> MLIRRLKDARLRAGISQEKLGVLAGIDEASASARMNQYEKGKHAPDFEMANRLAKVLKIPVSYLYTPEDDLAQIILTWNELNEQERKRINFYIRKKAK

Controller proteins play a key role in the temporal regulation of gene expression in bacterial restriction–modification (R–M) systems and are important mediators of horizontal gene transfer. They form the basis of a highly cooperative, concentration-dependent genetic switch involved in both activation and repression of R–M genes. Here we present biophysical, biochemical, and high-resolution structural analysis of a novel class of controller proteins, exemplified by C.Csp231I. In contrast to all previously solved C-protein structures, each protein subunit has two extra helices at the C-terminus, which play a large part in maintaining the dimer interface.

The protein crystallised in two space groups: a monoclinic form (P21) and a cubic form (F4132). The calculated Matthews coefficients were 2.38 Å3 Da− 1 (one monomer in the asymmetric unit) and 2.01 Å3 Da− 1 (two monomers in the asymmetric unit) for the cubic and monoclinic structures, respectively. Thus, there is a crystallographic dyad between the two subunits in the cubic form, whereas the subunits are related by a noncrystallographic dyad in the monoclinic form. The following analysis is based on the cubic form of C.Csp231I. The total dimer interface area of C.Csp231I is 1410 Å2 compared to 1040 Å2 in C.Esp1396I and 710 Å2 in C.AhdI. The striking feature in C.Csp231I is not that the dimer interface is larger, but rather that 75% of the dimer interface is contributed by the extended C-terminal helical region (helices 6 and 7; residues 67–98). This is achieved by the interleaving of the final two helices from each monomer. In fact, the five-helix bundle that makes up the main conserved domain only creates 310 Å2 of buried surface area on its own. Surprisingly, this domain contains the only pair of interchain H-bonds (Ser62-Thr66); in contrast, C.AhdI and C.Esp1396I contain a total of four and five interchain H-bonds, respectively. The analysis of B-factors in the cubic crystal form of C.Csp231I reveals that the extended C-terminal region of the protein, comprising helices 6 and 7, is significantly more mobile than the rest of the structure.>[2x]MGKTNDWLDFDQLAEEKVRDALKPPSMY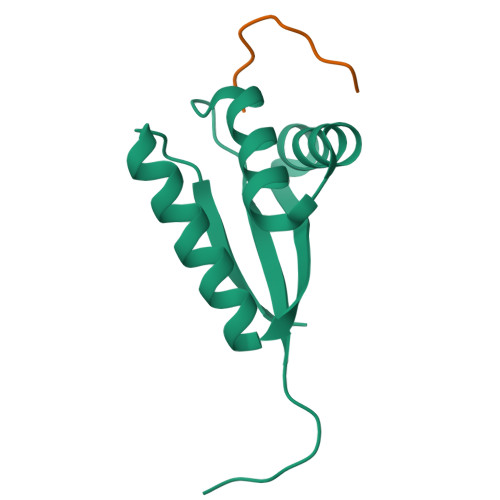KVILVNDDYTPMEFVIDVLQKFFSYDVERATQLMLAVHYQGKAICGVFTAEVAETKVAMVNKYARENEHPLLCTLEKAF;>[2x]FRSKGEELFT> YQD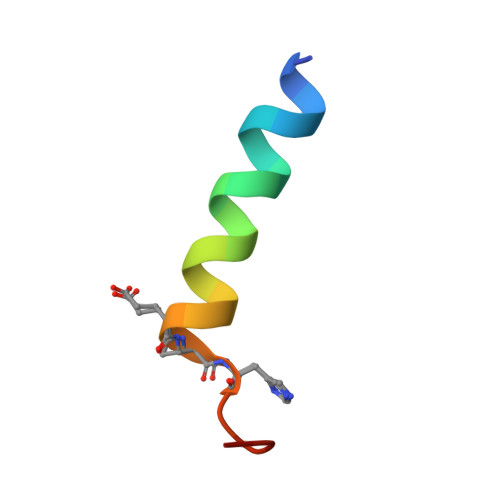LRRRFFLHHLIAEXHTAEIX>MMVISEKVRKALNDQLNREIYSSYLYLSMATYFDAEGFKGFAHWMKKQAQEELTHAMKFYEYIYKRGGRVELEAIEKPPSNWNGIKDAFEAALKHEEFVTQSIYNILELASEEKDHATVSFLKWFVDEQVEEEDQVREILDL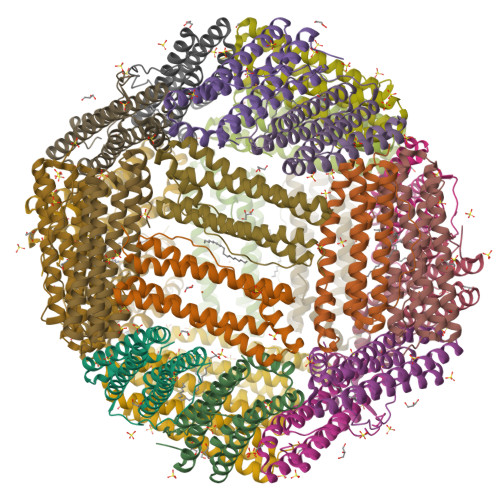LEKANGQMSVIFQLDRYLGQRE[8x]>STHYLAFPRASTITWGDDTRYWSWATVDFCSYAIEEARLLQVSWLDCRWSMDASDFKQDIWYNASVEV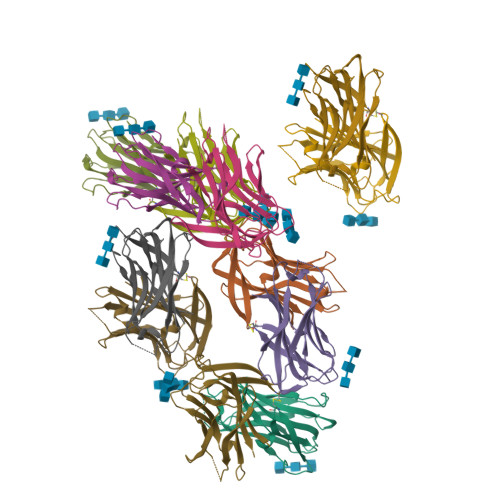MLTSNASGWNVPLHLEIELPDGSKQESQIVLAGRQPNVWFKIPIGKFILRGSLTSGTIRFGFYNHEGNWKRGLNIRTLAIQA[12x]> GAFLDKPKMEKHNAQGQGNGLRYGLSSMQGWRVEMEKAHTAVIGLPSGLESWSFFAVYDGHAGSQVAKYCCEHLLDHITNNQDFKGSAGAPSVENVKNGIRTGFLEIDEHMRVMSEKKHGADRSGSTAVGVLISPQHTYFINCGDSRGLLCRNRKVHFFTQDHKPSNPLEKERIQNAGGSVMIQRVNGSLAVSRALGDFDYKCVHGKGPTEQLVSPEPEVHDIERSEEDDQFIILACDGIWDVMGNEELCDFVRSRLEVTDDLEKVCNEVVDTCLYKGSRDNMSVILICFPNAPKVSPEAVKKEAELDKYLECRVEEIIKKQGEGVPDLVHVMRTLASENIPSLPPGGELASKRNVIEAVYNRLNPY

The PP2Cα is the prototype PP2C family phosphatase for which the catalytic mechanisms and cellular functions have been well characterized. The active site of PP2C is located at a cleft between two central β sheets, and it harbors a binuclear metal ion site required for catalysis. In the crystal structure of PP2Cα, the M2 metal ion is directly coordinated to the primary chain carbonyl of the Gly61 and the side-chain carboxylate group of Asp60. In addition to these direct interactions, the M2 metal ion of PP2Cα also indirectly interacts with Glu37 and Asp38 through water-mediated hydrogen bonds.

To reverse the negative charge of the D38, we also made a D38K mutant to see the mutating effect. To further elucidate the structural basis of the impaired function and catalysis of D38 mutants, we solved the crystal structures of PP2Cα-D38A and D38K with Mn2+ at 2.0 Å and 1.85 Å, respectively, and compared these structures with the PP2Cα-WT that was crystallized under similar conditions (1.95 Å). In addition, the electron density for the side chains of D38, A38 and the partial side chain of K38 are also unambiguously assigned in the PP2Cα-WT, PP2Cα-D38A and D38K crystal structures, respectively. However, in contrast to the crystal structure of the PP2Cα-WT, the electron density for the M2 metal ion and the phosphate can't be clearly located in the D38A or D38K crystal structures. In the crystal structure of the D38K mutant, the bridging water between the M2 metal ion and the D38 in the PP2Cα-WT was pushed outward by 0.7 Å because of the longer K38 side chain. The relocated water (WAT145) forms a hydrogen bond with the side chain of K38, which disabled M2 metal ion binding. Therefore, the crystal structures of PP2Cα-D38 mutants revealed that the D38A or D38K mutants of PP2Cα abolished the M2 metal ion binding by altering the H-bond network of the PP2Cα active site. However, the overexpression of an equal amount of PP2Cα-D38A mutant as the wild type only slightly decreased the EGF-induced ERK phosphorylation, and the overexpression of the PP2Cα-D38K mutant has little effect on the ERK phosphorylation increase. Accordingly, the D38A decreased sulfate binding by 4-fold, and D38K decreased the sulfate binding by 10-fold. However, the basic limbs of the D38A and D38K catalyzed pNPP hydrolysis were flat, suggesting an inefficient general acid catalysis for these two mutations.> GSHMSREEIRKVV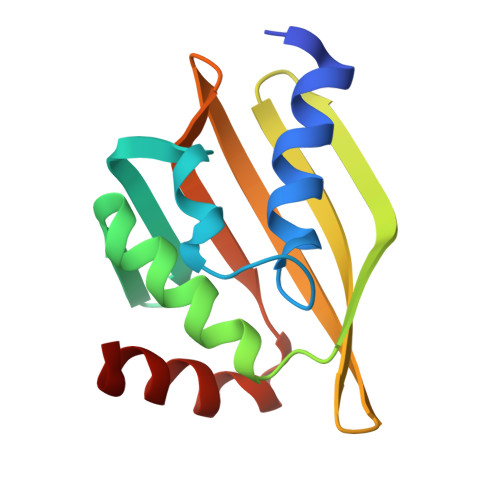EEMVRKLKQGSPEDISKYLSPDVRLEVGNYTFEGSEQVTKFWRMLTKFVDRVEVRKVQVDGNHVRVEVEVEWNGKKWTFEVEVEVRNGKIKRIRLQVDPEFKKVVQNIWNLL> GPLGSASLFATITGASKTEWSFSDIELTYRPDTLLSLGVMEFTLPSGFTANTKDTMNGNALRTTQILNNGKTVRVPLALDLLGAGEFKLKLNNKTL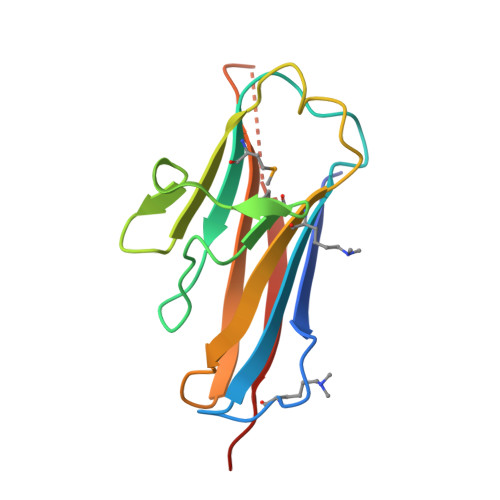PAAGTYTFRAENKSLSIGNKFYAEASIDVAKRST miniSOG (for mini Singlet Oxygen Generator)1 is a 106 amino acid flavin-binding protein that generates 1O2 under exposure to blue light. It was originally developed by Shu and coworkers for correlative light and electron microscopy (CLEM) as it both fluoresces and catalyzes the photo-oxidation of diaminobenzidine (DAB), providing high-resolution images. Novel applications are being actively developed since. miniSOG was engineered from the LOV2 (Light, Oxygen and Voltage) domain of Arabidopsis thaliana phototropin 21. The absence of a structure of miniSOG so far had prevented to rationalize these observations, which we have attempted here using a combined structural and photophysical approach.

Blue-light (440 nm) irradiation of a miniSOG crystal at 10 W·cm−2 led to a five-fold decrease of the fluorescence signal over a 30 min course and was gentle enough to keep diffraction around 2.0 Å resolution while affecting a sufficient fraction of molecules so that structural alterations could be visualized in electron density maps. A difference Fourier map calculated from non-irradiated and irradiated parts of a crystal revealed the loss of electron density all along the ribityl tail of the FMN, strongly suggesting its cleavage. Indeed, the 2Fobs − Fcalc electron density map of blue-light irradiated miniSOG reveals the unambiguous oxidation of three surface residues during irradiation. Tyr73 has been partially converted to a γ-peroxotyrosine. The loss of electron density on Trp81 is compatible with the formation of N-formylkynurenine (NFK), a well-known tryptophan oxidation product. Finally, His85 can be modeled by either a singly, or a doubly oxidized histidine, namely 2-oxo-histidine and 2,4-dioxo-histidine. Oxidation of Tyr73, His85 and Trp81 eliminates potential quenchers of 3miniSOG*, thereby decreasing the value of kp. Prolonged irradiation to blue light leads to several structural alterations of miniSOG, which include photodegradation of FMN into LC and oxidation of the quenching side chains. Formation of LC liberates the access of molecular oxygen to the alloxazine ring and reduces protein quenching of the triplet state, while oxidized electron-rich side chains cannot quench the triplet state of the chromophore. All this results in an increase of Φ∆ when photoconverted miniSOG is excited at the wavelengths where the formed LC absorbs.

> MEKSFVITDPRLPDNPIIFASDGFLELTEYSREEILGRNGRFLQGPETDQATVQKIRDAIRDQREITVQLINYTKSGKKFXNLLHLQPMRDQKGELQYFIGVQLDGEFIPNPLLG>MSDKDSKNTPQVPEKLGLSRRGFLGASAVTGAAVAATALGGAVMTRESWAQAVKESKQKIHVGPGELDDYYGFWSGGHQGEVRVLGVPSMRELMRIPVFNVDSATGWGLTNESRHIMGDSAKFLNGDCHHPHISMTDGKYDGKYLFINDKANSRVARIRLDIMKCDKMITVPNVQAIAGLRLQKVPHTKYVFANAEFIIPHPNDGKVFDLQDENSYTMYNAIDAETMEMAFQVIVDGNLDNTDADYTGRFAAATCYNSEKAFDLGGMMRNERDWVVVFDIHAVEAAVKAGDFITLGDSKTPVLDGRKKDGKDSKFTRYVPVPKNPHGCNTSSDGKYFIAAGKLSPTCSMIAIDKLPDLFAGKLADPRDVIVGEPELGLGPLHTTFDGRGNAYTTLFIDSQVVKWNMEEAVRAYKGEKVNYIKQKLDVHYQPGHLHASLCETNEADGKWLVALSKFSKDRFLPVGPLHPENDQLIDISGDEMKLVHDGPTFAEPHDCIMARRDQIKTKKIWDRNDPFFAPTVEMAKKDGINLDTDNKVIRDGNKVRVYMTSMAPAFGVQEFTVKQGDEVTVTITNIDQIEDVSHGFVVVNHGVSMEISPQQT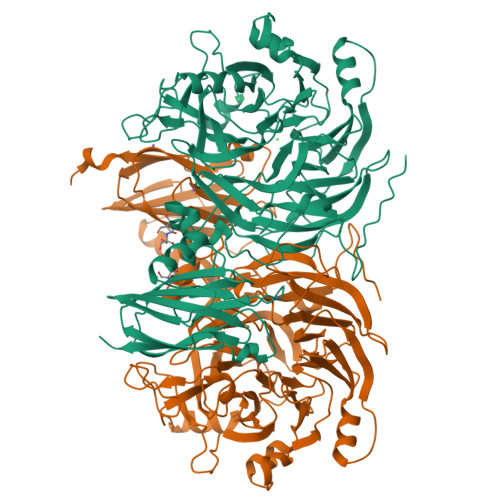SSITFVADKPGLHWYYCSWFCHALHMEMVGRMMVEPAWSHPQFEK[2x]> METACERLHVAQETQMQLIEKSSDKLQDHILYWTAVRTENTLLYAARKKGVTVLGHCRVPHSVVCQERAKQAIEMQLSLQELSKTE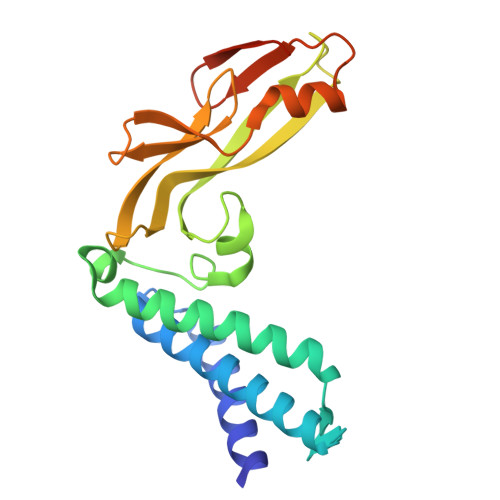FGDEPWSLLDTSWDRYMSEPKRCFKKGARVVEVEFDGNASNTNWYTVYSNLYMRTEDGWQLAKAGADGTGLYYCTMAGAGRIYYSAFGDEAARFSTTGHYSVRDQDRVYAGVSSTSSDFRDRP>[2x]MSVHV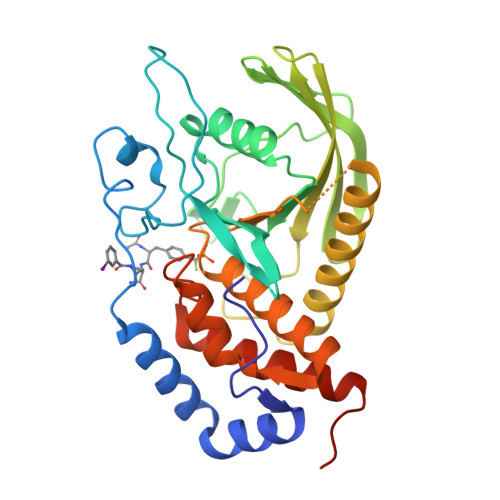PGPHAMTIQELVDYVNARQKQGIYEEYEDIRRENPVGTFHCSMSPGNLEKNRYGDVPCLDQTRVKLTKRSGHTQTDYINASFMDGYKQKNAYIGTQGPLENTYRDFWLMVWEQKVLVIVMTTRFEEGGRRKCGQYWPLEKDSRIRFGFLTVTNLGVENMNHYKKTTLEIHNTEERQKRQVTHFQFLSWPDYGVPSSAASLIDFLRVVRNQQSLAVSNMGARSKGQCPEPPIVVHCSAGIGRTGTFCSLDICLAQLEELGTLNVFQTVSRMRTQRAFSIQTPEQYYFCYKAILEFAEKEGMVSAHHHHHH> GGMQADKCPVTGATATTARGDSVEFDFFAAPQAYRRVAAEHARDGAFHSSRGDSFWVLSTYEGICAAFRDEDTFSVSRVSAADG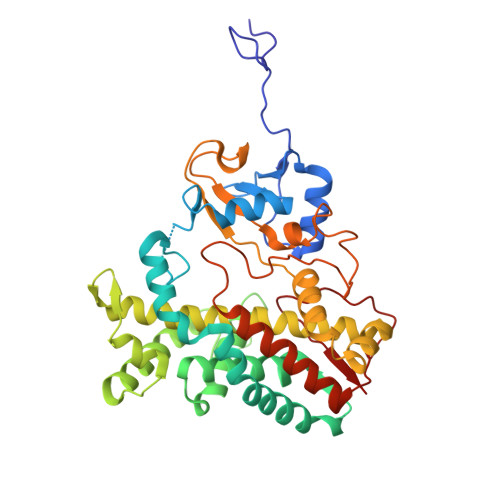AEDERWIPLTIQGRTHNEWRRRLAAWFTPQRARDLTPAIRANARRRISAFVDRGEVSFSDEFARPYVLENLMLAVGWPLADLDHLLAINVAMIRSREAPDPRQAFNAETAFPALQEYVRRHVARRRAEPVEGDLTSATFDWEIDGTPVSDADRESLLTVLFLAGVDSTVNHMANGIQHLAHHPGDRHRFLRDPEVRPAAVEEFLRVNSCMYPGRLATREGAGGVASQGDTVLLPLALANYDPAVFPEPERVDFDREQNPHIAFGTGHHQCLGAAYARAQILTAWEEWHELIPDYRLPDPTVEPPFLRNVYDLRIVW>GAMGIRNSMGQEPRTLPPSPNWYCARCSDAVPGGLFGFAARTSVFLVRVGPGAGESPGTPPFRVIGELVGHTERVSGFTFSHHPGQYNLC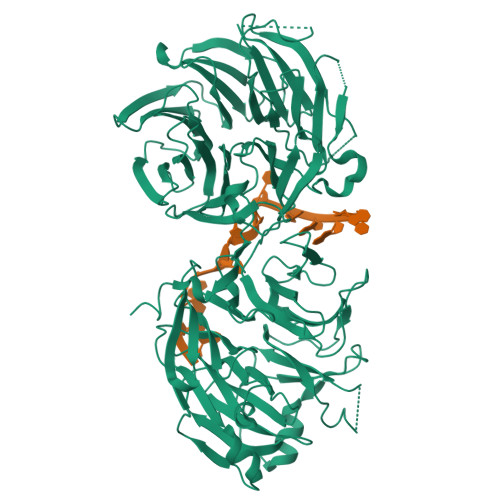ATSSDDGTVKIWDVETKTVVTEHALHQHTISTLHWSPRVKDLIVSGDEKGVVFCYWFNRNDSQHLFIEPRTIFCLTCSPHHEDLVAIGYKDGIVVIIDISKKGEVIHRLRGHDDEIHSIAWCPLPGEDCLSINQEETSEEAEITNGNAVAQAPVTKGCYLATGSKDQTIRIWSCSRGRGVMILKLPFLKRRGGGIDPTVKERLWLTLHWPSNQPTQLVSSCFGGELLQWDLTQSWRRKYTLFSASSEGQNHSRIVFNLCPLQTEDDKQLLLSTSMDRDVKCWDIATLECSWTLPSLGGFAYSLAFSSVDIGSLAIGVGDGMIRVWNTLSIKNNYDVKNFWQGVKSKVTALCWHPTKEGCLAFGTDDGKVGLYDTYSNKPPQISSTYHKKTVYTLAWGPPVPPMSLGGEGDRPSLALYSCGGEGIVLQHNPWKLSGEAFDINKLIRDTNSIKYKLPVHTEISWKADGKIMALGNEDGSIEIFQIPNLKLICTIQQHHKLVNTISWHHEHGSQPELSYLMASGSNNAVIYVHNLKTVIESSPESPVTITEPYRTLSGHTAKITSVAWSPHHDGRLVSASYDGTAQVWDALREEPLCNFRGHRGRLLCVAWSPLDPDCIYSGADDFCVHKWLTSMQDHSRPPQGKKS[2x]(2~{S})-2-[[5-azanyl-1-[(2~{R},3~{R},4~{S},5~{R})-3,4-bis(oxidanyl)-5-(phosphonooxymethyl)oxolan-2-yl]imidazol-4-yl]carbonylamino]butanedioic acid | C13 H19 N4 O12 P | 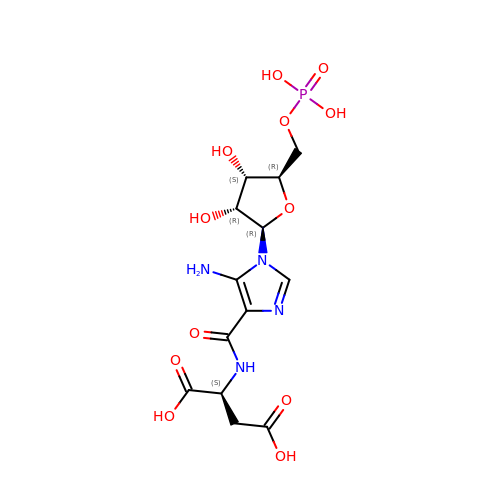NAQGHJTUZRHGAC-ZZZDFHIKSA-N>[4x]GAMGSEQRASLDSEESESPPQENSCLDPPDRDPNCKPPPVKPHIFTTRSRTRLFGKGDSEEASPLDCPYEEGGLASCPIITVSSVLTIQRPGDGPASVRPSSQDSVSAGEKPPRLYDRRSIFDAVAQSNCQELESLLPFLQRSKKRLTDSEFKDPETGKTCLLKAMLNLHNGQNDTIALLLDVARKTDSLKQFVNASYTDSYYKGQTALHIAIERRNMTLVTLLVENGADVQAAANGDFFKKTKGRPGFYFGELPLSLAACTNQLAIV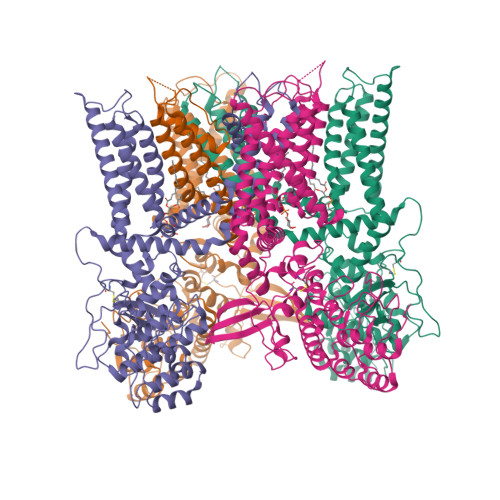KFLLQNSWQPADISARDSVGNTVLHALVEVADNTVDNTKFVTSMYNEILILGAKLHPTLKLEEITNRKGLTPLALAASSGKIGVLAYILQREIHEPECRHLSRKFTEWAYGPVHSSLYDLSCIDTCEKNSVLEVIAYSSSETPNRHDMLLVEPLNRLLQDKWDRFVKRIFYFNFFVYCLYMIIFTAAAYYRPVEGLPPYKLKNTVGDYFRVTGEILSVSGGVYFFFRGIQYFLQRRPSLKSLFVDSYSEILFFVQSLFMLVSVVLYFSQRKEYVASMVFSLAMGWTNMLYYTRGFQQMGIYAVMIEKMILRDLCRFMFVYLVFLFGFSTAVVTLIEDGKNNSLPMESTPHKCRGSACKPGNSYNSLYSTCLELFKFTIGMGDLEFTENYDFKAVFIILLLAYVILTYILLLNMLIALMGETVNKIAQESKNIWKLQRAITILDTEKSFLKCMRKAFRSGKLLQVGFTPDGKDDYRWCFRVDEVNWTTWNTNVGIINEDPGNCEGVKRTLSFSLRSGRVSGRNWKNFALVPLLRDASTRDRHATQQEEVQLKHYTGSLKPEDAEVFKDSMVPGEK>[4x]CLTSCPPLWTGFNGKCFRLFHNHLNFDNAENACRQFGLASCSGDELATGHLASIHSAESQAFLTELVKTSLPDLITGGWAPQVYIGMKVGSTNSDQTWTDGSSVDYDGWVSGEPNN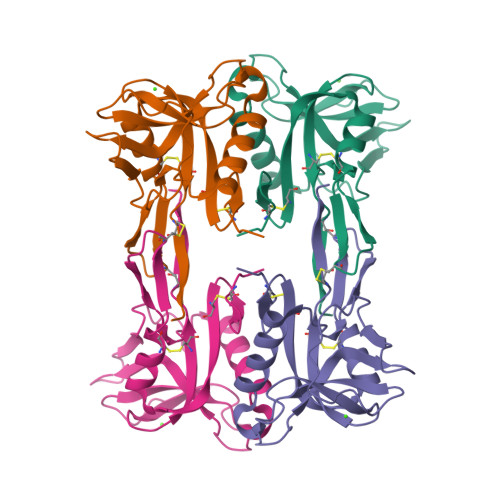GPNSRGAIAAGDYSRGFWADVYSNNNFKYICQLPCVHYTLE> MSLQQALIVEDYQAAAETFKELLEMLGFQADYVMSGTDALHAMSTRGYDAVFIDLNLPDTSGLALVKQLRALPMEKTSKFVAVSGFAKNDLGKEACE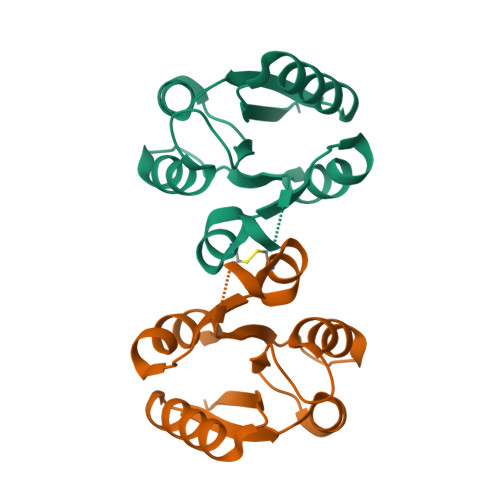LFDFYLEKPIDIASLEPILQSIEGHHHHHH N-(1-benzoyl-1,2,3,4-tetrahydroquinolin-6-yl)-2-(3-cyano-2-methoxyphenyl)acetamide | C26 H23 N3 O3 | 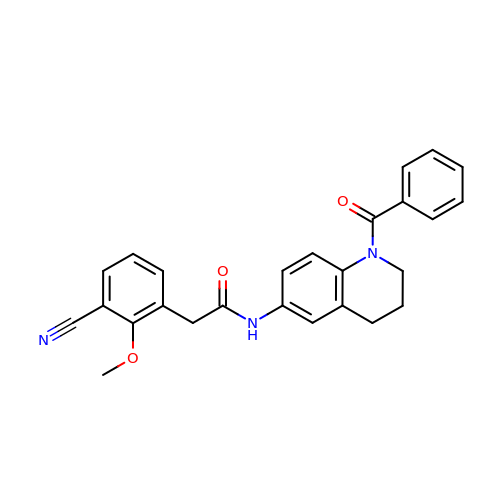FBPFRQJGDYZWBK-UHFFFAOYSA-N(1R)-1,5-anhydro-1-(5-methyl-1,3,4-oxadiazol-2-yl)-D-glucitol | C9 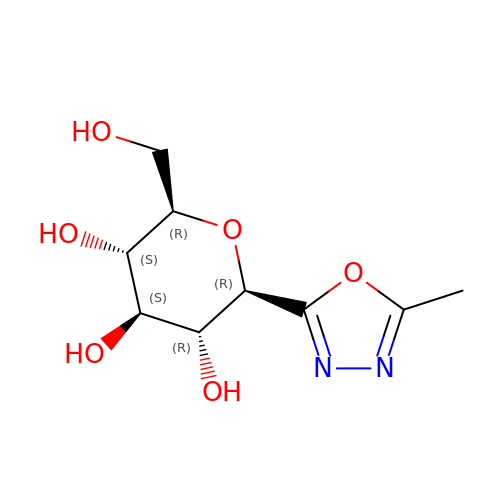H14 N2 O6 | HCSFWJQLIPWUFZ-JAJWTYFOSA-N> SAGMVVFIDPGHNGANDASIGRQVPTGRGGTKNCQASGTSTNSGYPEHTFTWETGLRLRAALNALGVRTALSRGNDNALGPCVDERANMANALRPNAIVSLHADGGPASGRGFHVNYSAPPLNAIQAGPSVQFARIMRDQLQASGIPKANYIGQDGLYGRSDLAGLNLAQYPSILVELGNMKNPADSALMESAEGRQKYANALVRGVAGFLATQGQAR

Amidases, also known as N-acetylmuramyl-l-alanine hydrolases, break the bond between the L-Ala and NAM, separating the peptide stem from the linear glycan chain. Gene analysis of M. tuberculosis revealed the presence of four amidase homologues: Ami1 (Rv3717), Ami2/CwlM (Rv3915), Ami3 (Rv3811), and Ami4 (Rv3594).12 However, the functions of Ami3 and Ami4 remain unknown. The crystal structure of Ami1 has been solved, and its PG hydrolase activity has been demonstrated in vitro. Furthermore, Ami1 is specifically required in M. tuberculosis during chronic mouse infection, as its amidase activity contributes to the pathogens ability to persist within the host.

In this work, we obtained the 3-D structure of the Ami1-5 complex at atomic resolution (1.45 Å). Compound 5 was localized within the catalytic groove, positioned at 4.3 Å from residue His125, which is part of the coordination triad responsible for binding Zn2+, along with residues His35 and Glu70 in the active site. Compound 5 is positioned within a hydrophobic core composed of residues Leu186, Leu189, Leu197 and Leu198, Val186, Ala187, Gly188 and Ile121. The phenyl ring is stabilized by π–alkyl interactions with Leu189 and Leu198, and van der Waals interactions with Asp32, Ile121, Ser123, and Ser196. The tetrazole ring is stabilized by Val106 (which adopts a double conformation) through a π–σ interaction, π–alkyl interactions with Leu196 and Leu198, and hydrogen bonds formed with the main chain of Gly188 and three water molecules. Finally, the iodine atom engages in an alkyl interaction with residue Arg109. Interestingly, a network of water-mediated interactions stabilizes the tetrazole ring of compound 5. These water molecules are positioned in the catalytic site, between the hydrophobic core and the coordination zinc triad. There is only a 0.7 Å distance between a nitrogen atom (N06) of the tetrazole ring in compound 5 and an oxygen atom (0 × 101) of iso-d-glutamine. This suggests that the presence of compound 5 in the cavity may hinder substrate binding, and, consequently, inhibit the hydrolysis reaction.> SDKKTLNDNRSHHDFTAGEKINYSIETVVPWNIANKKVYTITDNPSKGLIMDADTIQIEGLASNKYTVKKNADNGFTITIPAANLAAFAGKTLKTTVKGHLSIEDLTLIDTGIPNKATAKVDNEAHHEVKSEEVFTGGKKFVKVDGSNQSKTLAGAQFQLVIVKNGQVVKYAHGNEKDGYTFDTNNTNVATKTTGENGQFEFAGLKYSESLEAGESYAVKEVKAPTGYDLLKDPVLFTVTKDSYKTVQ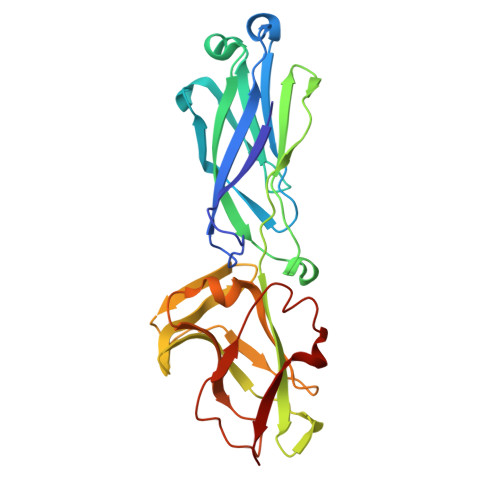AADGQKISNTK>[6x]MGHHHHHHHHEFIPSNTDYPGPHHFEVTFQQSSTAKSATWTYSPLLKKLYCQIAKTCPIQIKVSTPPPPGTAIRAMPVYKK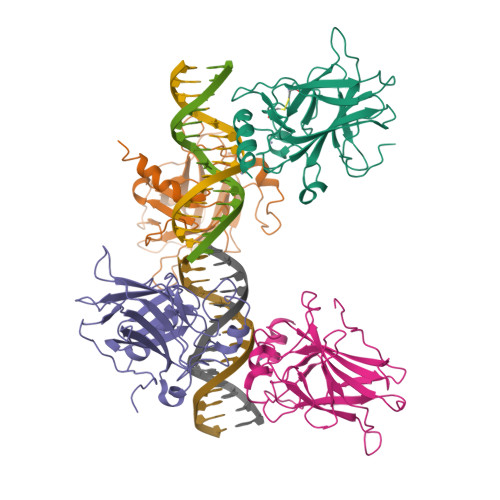AEHVTDVVKRCPNHELGRDFNEGQSAPASHLIRVEGNNLSQYVDDPVTGRQSVVVPYEPPQVGTEFTTILYNFMCNSSCVGGMNRRPILIIITLEMRDGQVLGRRSFEGRICACPGRDRKADEDHYREQ>AEVGSVIGASLFDQLLKHRNDQACEGKGFYSYNAFITAARSFAAFGTTGDSNTRKREVAAFLAQTSHETTGGAATSPDGPYAWGYCFVTERDKSNRYCDGSGPCSAGKSYYGRGPIQLTHNYNYNAAGRALGVDLINNPDLVARDAVVSFKTALWFWMTPQGNKPSCHDVITNRWTPSAADK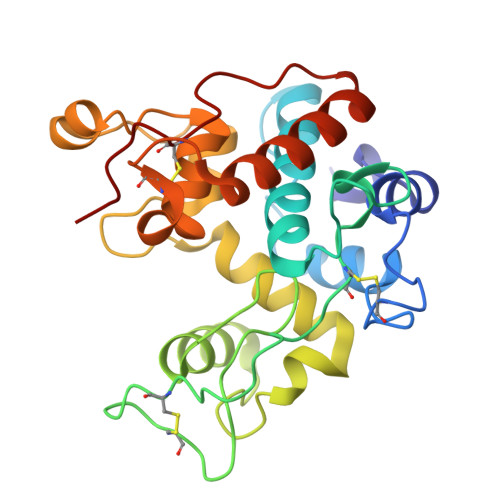AANRVPGFGVITNIINGGLECGKGPTPASGDRIGFYKRYCDVFGVSYGPNLNCRDQRPFG[2x]>[8x]MNEAIRTIQDHRSIRQYTDEAVSDEHLDTIIQSAQSAASSINGQQVTIISVQDKEKKKKLSELAGNQAWIDQAPLFLIFCADFNRAKIAAELNDAPLGVT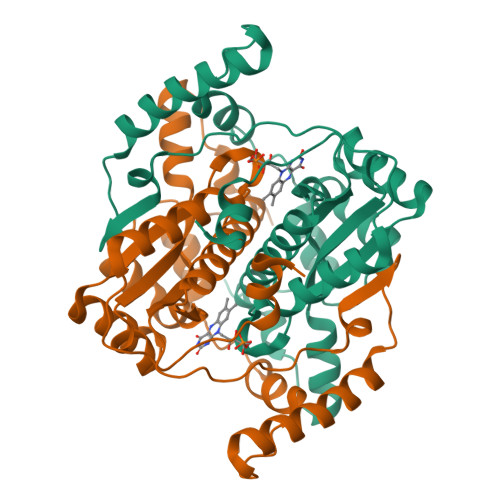DGLESILVGATDAGISLEAATVAAESLGLGTVPIGGIRRKPLEVIELLDLPEYVFPVSGLVVGHPSDHSAKKPRLPQAAVHHRESYNHDLKSLIQDYDAEMAEYMKKRTNGADDRNWSQTVSAIYKTIYYPEVRAMLEKQGFKFEKGHHHHHH> MGSSHHHYHHENLYFQGSNIAFYVVSDVHGYIFPTDFTSRNQYQPMGLLLANHVIEQDRRQYDQSFKIDNGDFLQGSPFCNYLIAHSGSSQPLVDFYNRMAFDFGTLGNHEFNYGLPY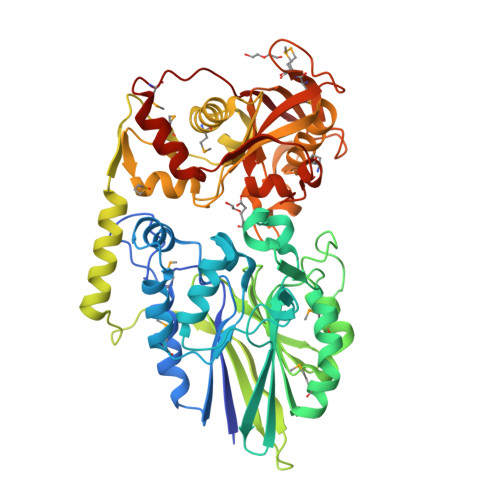LKDTLRRLNYPVLCANIYENDSTLTDNGVKYFQVGDQTVGVIGLTTQFIPHWEQPEHIQSLTFHSAFEILQQYLPEMKRHADIIVVCYHGGFEKDLESGTPTEVLTGENEGYAMLEAFSKDIDIFITGHQHRQIAERFKQTAVIQPGTRGTTVGRVVLSTDEYENLSVESCELLPVIDDSTFTIDEDDQHLRKQLEDWLDYEITTLPYDMTINHAFEARVAPHPFTNFMNYALLEKSDADVACTALFDSASGFKQVVTMRDVINNYPFPNTFKVLAVSGAKLKEAIERSAEYFDVKNDEVSVSADFLEPKPQHFNYDIYGGVSYTIHVGRPKGQRVSNMMIQGHAVDLKQTYTICVNNYRAVGGGQYDMYIDAPVVKDIQVEGAQLLIDFLSNNNLMRIPQVVDFKVEK4-(4-{[(2-chloro-6-fluorophenyl)carbamoyl]amino}-1H-pyrazol-1-yl)-5-methyl-N-(oxetan-3-yl)thiophene-2-carboxamide | C19 H17 Cl F 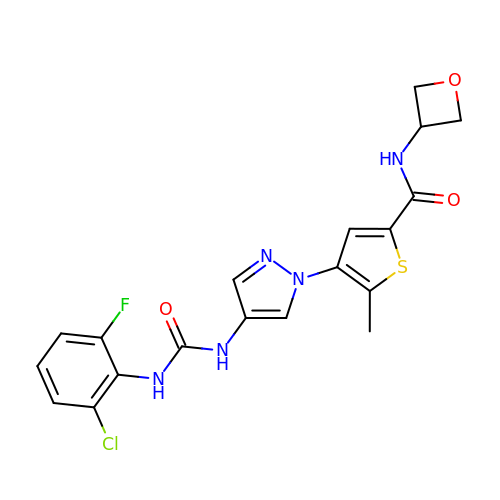N5 O3 S | JRCVTCDIBTUNEL-UHFFFAOYSA-N> 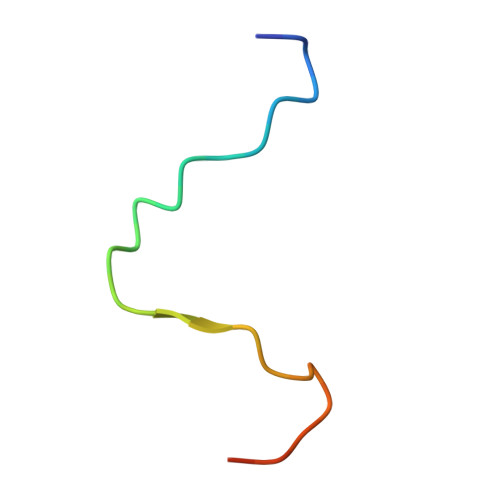YTEFAPPPTPMVDHLVASNPFEDDFGA CCs are quaternary structures comprising two or more α-helices supercoiled around each other with cyclic (Cn) or dihedral (Dn) symmetry. Here, we describe variants with all combinations of the aliphatic residues, Ile, Leu and Val, at a and d to give four classes of peptide: the ββ class, with a and d = Ile or Val; Lβ, a = Leu and d = Ile or Val; βL, a = Ile or Val and d = Leu; and LL, a = d = Leu. Peptides are named systematically appending the one-letter code for the amino acids at the a and d sites to “CC-Type2-“; e.g., CC-Hept becomes CC-Type2-LI. In summary, solution-phase data and X-ray crystal structures demonstrate conclusively that different classes of Type-2 coiled-coil (CC) peptides—i.e., based on abcdefg repeats with predominantly hydrophobic residues at a, d, e and g—adopt a range of distinct states.

To explore this switch between assembling open α-helical barrels and collapsed CCs, we tested if examples of some of the latter could be opened by introducing polar residues into the hydrophobic repeats of βL and LL sequences. Specifically, we mutated the centremost Leu at d (position 17) to Glu to give CC-Type2-IL-Sg-L17E and CC-Type2-LL-L17E. However, unlike the parents, they had accessible thermal unfolding transitions. Both transitions were pH dependent with stabilities increasing sharply below pH 6–7. Neither of the L17E peptides bound DPH, but both sequestered its cationic derivative trimethyl-ammonium DPH (TMA-DPH) with μM affinities suggesting that the barrel states are accessible. Surprisingly, the X-ray crystal structure of CC-Type2-LL-L17E overlaid almost perfectly with that for the parent CC-Type2-LL; i.e., all six Glu-17 side chains are completely buried within the core of the assembly. The experimental and computational data correlated well: For CC-Type2-LL-L17E, at pH 3–6 experimentally the peptide was highly thermally stable, and simulations showed a mixed population of singly and doubly charged states; from pH 6–7 the thermal stability of the peptide decreased, and the main charge states were (Glu-17)62- and (Glu-17)63-; and above pH 8, both the α-helicity and the thermal stability decreased dramatically, and more than half of the Glu residues were deprotonated. Thus, CC-Type2-LL-L17E appears to tolerate two buried charged Glu residues, but above this number severely destabilises the structure. The macroscopic pKa for the transition from two to three buried charges was calculated as 6.8, which is > 2 pH units above free Glu and considered highly perturbed.

>XGELAQALKELAKALKEEAWALKELAQALKGX[24x]>GSHMASASMKFAVIDRKNFTLIHFEIEKPIKPEILKEIEIPSVDTRKGVVISGRGPMWMHCFLAHKYHHTPFVAVYDPRLGAVVVQSHSELREGDVIDV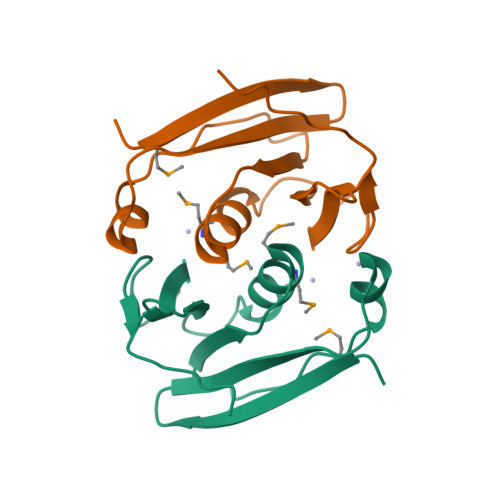VVEEILKGGVRHV[2x]> NDPESALNRAVGRVADTVASGPVNTEQIPALTAVETGHTSQVVPSDTMQTRHVINYHTRSESSIENFMGRAACVYIAQYATEKVNDELDRYTNWEITTRQVAQLRRKLEMFTYMRFDLEITFVITSSQRTSTTYASDSPPLTHQVMYVPPGGPIPKSYEDFAWQTSTNPSVFWTEGNAPPRMSIPFMSVGNAYCNFYDGWSHFSQSGVYGYTTLNNMGHLYFRHVNKSTAYPVNSVARVYFKPKHVKAWVPRAPRLCPYLKARNVNFNVQGVTESRNKITLDRSTHNPLANT;> SPTVEECGYSDRVRSITLGNSTITTQECANVVVGYGVWPTYLSDHEATAVDQPTQPDVATCRFYTLESVKWESSSAGWWWKFPEALSDMGLFGQNMQYHYLGRTGYTIHVQCNASKFHQGCLLVVCVPEAEMGAATTDHAFNHTKLSNIGQAMEFSAKKSTDQTGPQTAVHNAGMGVAVGNLTIFPHQWINLRTNNSATIVMPYINSVPMDNMYRHYNFTLMVIPFAKLEHSPQASTYVPITVTVAPMCAEYNGLRLAGHQ;> GLPTMNTPGSTQFLTSDDFQSPSAMPQFDVTPEIQIPGQVRNLMEIAEVDSVVPVNNTEGHVNSMEAYRIPVRPQTSSGEQVFGFQLQPGHDSVLKHTLLGEILNYYANWSGSMKLTFMYCGAAMATGKFLIAYSPPGAGVPGSRRDAMLGTHVIWDVGLQSSCVLCVPWISQTNYRYVTSDAYTDAGYITCWYQTSIVTPPDIPTTSTILCFVSACNDFSVRLLRDTPFITQQALFQ;> XGAQVSTQKTGAHETGLNASGNSIIHYTNINYYKDSASNSLNRQDFTQDPSKFTEPVKDVMIKTLPALN

The genus Enterovirus within the Picornaviridae, a family of non-enveloped viruses with a positive single-stranded RNA genome, is comprised of more than 100 serotypes. Human enteroviruses (EV) are presently classified into four groups, Enterovirus A-D (EV-A, B, C, and D), among which EV-B, the largest group, consists of over 60 serotypes, including all 6 serotypes of coxsackievirus B (CVB1-6), coxsackievirus A9 (CVA9), over 30 serotypes of echoviruses and more than 20 newly identified enteroviruses. The capsid proteins (VP1, VP2, and VP3) adopt the classical eight-stranded anti-parallel β-barrel configuration with the N-termini residing inside and the C-termini exposed on the surface. Most of the uncoating receptors bind to the “canyon” sites of the viral particle, dislodging the “pocket factor” in VP1 and subsequently triggering conformational changes of the intact particle to release the genome, albeit that SCARB2 binds EV71 outside the canyon.

Here we report the structural characterizations of E30 E-particle, A-particle and mature virion, among which E-particle and mature virion are compact with fully ordered epitopes, showing the potential to be ideal vaccine candidates. We separated out two distinct types of particles by ultracentrifugation and characterized them using SDS-PAGE, single-stranded RNA detection and analytical ultracentrifugation as either 143S F-particles, containing RNA and a full complement of proteins VP1–VP4, or 80S E-particles containing VP0, VP1, and VP3. The three types of particles reveal a pseudo T = 3 symmetry arrangement and the overall structures of three particles resemble those of other EVs. Like other EVs, E30 contains the canyon-like depression and the hydrophobic pocket in VP1 harboring a pocket factor beneath the depression. Like most enteroviruses, E30 F-particle possesses the hydrophobic pocket in VP1 harboring a pocket factor, whereas both E- and A-particles lack hydrophobic pocket and harbor no pocket factor. However, compared with EV-As and EV-Cs, which have a continuous circular canyon around each five-fold mesa, in EV-Bs, there are, instead, five distinct ~15-Å deep depressions. A ridge between each depression is formed by the C-termini of VP1 and VP3. A number of key structural elements contributing to the canyon, including the VP1 BC loop (the north wall of the canyon), the VP2 EF loop (back part of the south wall) and significantly shortened VP1 GH loop (front part of the south wall) adopt different conformations and move toward the front, together with the ridges, ablating the back portion of the canyon. Superposition of the asymmetric units (protomers) verifies the similarity in capsid structures of the F- and E-particles (RMSD = 0.4 Å in Cα atoms).>[16x]MTTVSCPANVITTTESDRIAGLFNIPAGIIPTGNVLSTIEVCAHRCIFDFFKQIRSDDNSLYSAQFDILLGTYCNTLNFVRFLELGLSVACICTKFPELAYVRDGVIQFEVQQPMIARDGPHPVDQPVHNYMVKRIHKRSLSAAFAIASEALSLLSNTYVDGTEIDSSLRIRAIQQMARNLRTVLDSFERGTADQLLGVLLEKAPPLSLLSPINKFQPEGHLNRVARAALLSDLKRRVCADMFFMTRHAREPRLISAYLSDMVSCTQPSVMVSRITHTNTRGRQVDGVLVTTATLKRQLLQGILQIDDTAADVPVTYGEMVLQGTNLVTALVMGKAVRGMDDVARHLLDITDPNTLNIPSIPPQSNSDSTTAGLPVNARVPADLVIVGDKLVFLEALERRVYQATRVAYPLIGNIDITFIMPMGVFQANSMDRYTRHAGDFSTVSEQDPRQFPPQGIFFYNKDGILTQLTLRDAMGTICHSSLLDVEATLVALRQQHLDRQCYFGVYVAEGTEDTLDVQMGRFMETWADMMPHHPHWVNEHLTILQFIAPSNPRLRFELNPAFDFFVAPGDVDLPGPQRPPEAMPTVNATLRIINGNIPVPLCPISFRDCRGTQLGLGRHTMTPATIKAVKDTFEDRAYPTIFYMLEAVIHGNERNFCALLRLLTQCIRGYWEQSHRVAFVNNFHMLMYITTYLGNGELPEVCINIYRDLLQHVRALRQTITDFTIQGEGHNGETSEALNNILTDDTFIAPILWDCDALIYRDEAARDRLPAIRVSGRNGYQALHFVDMAGHNFQRRDNVLIHGRPVRGDTGQGIPITPHHDREWGILSKIYYYIVIPAFSRGSCCTMGVRYDRLYPALQAVIVPEIPADEEAPTTPEDPRHPLHAHQLVPNSLNVYFHNAHLTVDGDALLTLQELMGDMAERTTAILVSSAPDAGAATATTRNMRIYDGALYHGLIMMAYQAYDETIATGTFFYPVPVNPLFACPEHLASLRGMTNARRVLAKMVPPIPPFLGANHHATIRQPVAYHVTHSKSDFNTLTYSLLGGYFKFTPISLTHQLRTGFHPGIAFTVVRQDRFATEQLLYAERASESYFVGQIQVHHHDAIGGVNFTLTQPRAHVDLGVGYTAVCATAALRCPLTDMGNTAQNLFFSRGGVPMLHDNVTESLRRITASGGRLNPTEPLPIFGGLRPATSAGIARGQASVCEFVAMPVSTDLQYFRTACNPRGRASGMLYMGDRDADIEAIMFDHTQSDVAYTDRATLNPWASQKHSYGDRLYNGTYNLTGASPIYSPCFKFFTPAEVNTNCNTLDRLLMEAKAVASQSSTDTEYQFKRPPGSTEMTQDPCGLFQEAYPPLCSSDAAMLRTAHAGETGADEVHLAQYLIRDASPLRGCLPLPR;>MTQPASSRVVFDPSNPTTFSVEAIAAYTPVALIRLLNASGPLQPGHRVDIA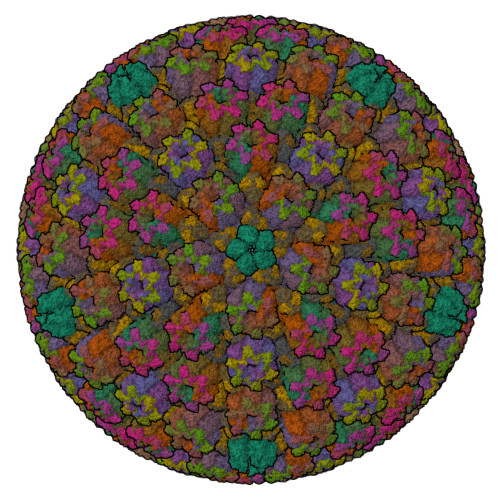DARSIYTVGAAASAARARANHNANTIRRTAMFAETDPMTWLRPTVGLKRTFNPRIIRPQPPNPSMSLGISGPTILPQKTQSADQSALQQPAALAFSGSSPQHPPPQTTSASVGQQQHVVSGSSGQQPQQGAQSSTVQPTTGSPPAAQGVPQSTPPPTQNTPQGGKGQTLSHTGQSGNASRSRRV[15x];>[10x]MAMPFEIEVLLPGELSPAETSALQKCEGKIITFSTLRHRASLVDIALSSYYINGAPPDTLSLLEAYRMRFAAVITRVIPGKLLAHAIGVGTPTPGLFIQNTSPVDLCNGDYICLLPPVFGSADSIRLDSVGLEIVFPLTIPQTLMREIIAKVVARAVERTAAGAQILPHEVLRGADVICYNGRRYELETNLQHRDGSDAAIRTLVLNLMFSINEGCLLLLALIPTLLVQGAHDGYVNLLIQTANCVRETGQLINIPPMPRIQDGHRRFPIYETISSWISTSSRLGDTLGTRAILRVCVFDGPSTVHPGDRTAVIQV;>[5x]MGSQPTNSHFTLNEQTLCGTNISLLGNNRFIQIGNGLHMTYAPGFFGNWSRDLTIGPRFGGLNKQPIHVPPKRTETASIQVTPRSIVINRMNNIQINPTSIGNPQVTIRLPLNNFKSTTQLIQQVSLTDFFRPDIEHAGSIVLILRHPSDMIGEANTLTQAGRDPDVLLEGLRNLFNACTAPWTVGEGGGLRAYVTSLSFIAACRAEEYTDKQAADANRTAIVSAYGCSRMETRLIRFSECLRAMVQCHVFPHRFISFFGSLLEYTIQDNLCNITAVAKGPQEAARTDKTSTRRVTANIPACVFWDVDKDLHLSADGLKHVFLVFVYTQRRQREGVRLHLALSQLNEQCFGRGIGFLLGRIRAENAAWGTEGVANTHQPYNTRALPLVQLSNDPTSPRCSIGEITGVNWNLARQRLYQWTGDFRGLPTQLSCMYAAYTLIGTIPSESVRYTRRMERFGGYNVPTIWLEGVVWGGTNTWNECYY>[2x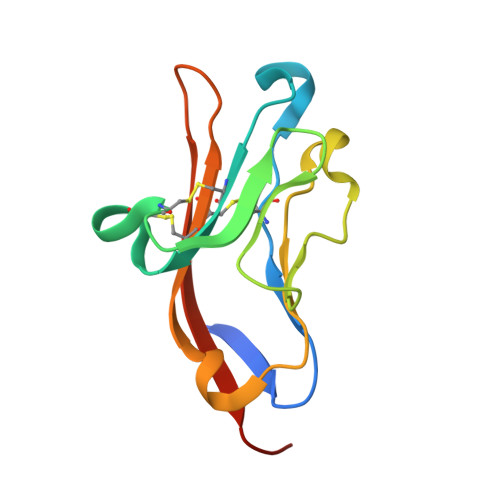]MESHTAVQGLAGHPVTLPCIYSTHLGGIVPMCWGLGECRHSYCIRSLIWTNGYTVTHQRNSRYQLKGNISEGNVSLTIENTVVGDGGPYCCVVEIPGAFHFVDYMLEVKPELVPR>[2x]EMCEIPEMDSHLVEKLGQHLLPWMDRLSLEHLNPSIYVGLRLSSLQAGTKEDLYLHSLKLGYQQCLLGSAFSEDDGDCQGKPSMGQLALYLLALRANCEFVRGHKGDRLVSQLKWFLEDEKRAIGHDHKGHPHTSYYQYGLGILALCLHQKRVHDSVVDKLLYAVEPFHQGHHSVDTAAMAGLAFTCLKRSNFNPGRRQRITMAIRTVQEEILKAQTPEGHFGNVYSTPLALQFLMTSPMRGAELGTACLKARVALLASLQDGAFQNALMISQLLPVLNHKTYIDLIFPDCLAPRVMLEPAAETIPQTQEIISVTLQVLSLLPPYRQSISVLAGSTVEDVLKKAHELGGFTYETQASLSGPYLTSVMGKAAGEREFWQLLRDPNTPLLQGIADYRPKDGETIELRLVSW;>[2x]SCPPTKFQCRTSGLCVPLTWRCDRDLDCSDGSDEEECRIEPCTQKGQCPPPPGLPCPCTGVSDCSGGTDKKLRNCSRLACLAGELRCTLSDDCIPLTWRCDGHPDCPDSSDELGCGTNE

Mammals depend on dietary uptake of Cobalamin (Cbl), which is a cofactor of at least two enzymes that are part of essential biochemical pathways. CD320 is a member of the Low-density Lipoprotein Receptor (LDLR) family, a large group of mostly multi-ligand receptors involved in cholesterol uptake and other physiologically essential functions. CD320 features an N-terminal, extracellular fragment comprising two LDLR type A (LDLR-A) domains separated by an epidermal growth factor (EGF) homology domain, the exact function of which has so far not been determined. While the majority of related LDLR domain-containing receptors bind multiple and distinct ligands, CD320 has been reported to bind TC with high specificity and affinity as evidenced by the lack of interference in TC binding from related LDLR ligands like LDL and RAP as well as high affinity for TC of both the full-length receptor and its soluble ectodomain81318.

Various CD320 truncations were generated and tested and a final crystallization construct comprising residues 53–199 of the extracellular domain of CD320 and TC residues 1–409 was chosen for structure determination. The TC-CD320 co-crystal structure, phased by molecular replacement using Cbl-bound TC as a search model, was refined to 2.1 Å resolution and revealed a 1:1 complex of TC-CD320. Whereas clear electron density was observed for LDLR-A1 residues 53–89 and LDLR-A2 residues 129-171, no density was observed for the EGF-like domain (residues 90–128). In agreement with epitope mapping studies, both LDLR-A1 and LDLR-A2 of CD320 exclusively interact with the α domain of TC. The structure of CD320-bound TC is very similar to that of its free state20 (r.m.s.d of all Cα atoms of 0.43Å) with a few key differences. The interface of TC and CD320 consists of ∼900 Å2 buried surface area, with LDLR-A2 contributing 486 Å2 compared with 405 Å2 for LDLR-A1. The fold of the LDLR-A domains of CD320 is similar to that of related family members. Both LDLR-A domains contain central Ca2+ ions bound by four conserved acidic residues and two backbone carbonyls in an octahedral coordination. In LDLR-A1, the Ca2+-coordinating carboxylate groups of Asp75 and Asp79 form salt bridges with Lys105 of TC, forming an ‘acidic necklace' previously found to be a key feature of LDLR/ligand complexes. The equivalent acidic necklace in LDLR-A2 is formed by Lys114 of TC and the Ca2+ coordinating carboxylate groups of Asp153 and Asp157 of CD320. LDLR-A1 contacts TC helices α3 and α5, whereas LDLR-A2 interacts with TC helix α5 and the loop between helices α6 and α7.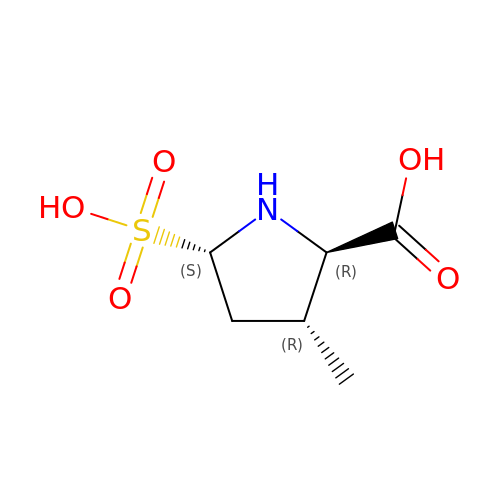3-METHYL-5-SULFO-PYRROLIDINE-2-CARBOXYLIC ACID | C6 H11 N O5 S | PZCKFQRRNSACOM-MROZADKFSA-N> PLTATVDGIIQPMLKAYRIPGMAVAVLKDGKAHYFNYGVANRESGQRVSEQTLFEIGSVSKTLTATLGAYAAVKGGFELDDKVSQHAPWLKGSAFDGVTMAELATYSAGGLPLQFPDEVDSNDKMQTYYRSWSPVYPAGTHRQYSNPSIGLFGHLAANSLGQPFEQLMSQTLLPKLGLHHTYIQVPESAMANYAYGYSKEDKP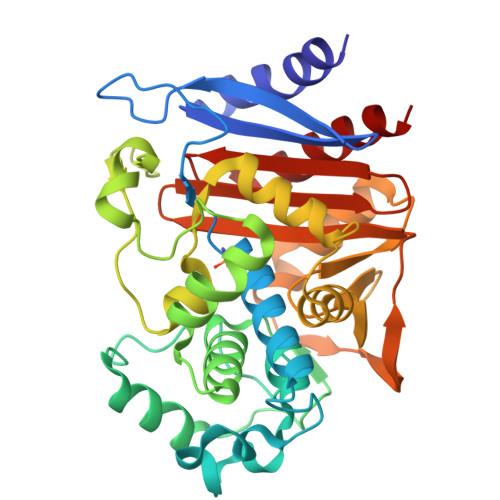IRATPGVLAAEAYGIKTGSADLLKFVEANMGYQGDAALKSAIALTHTGFHSVGEMTQGLGWESYDYPVTEQVLLAGNSPAVSFQANPVTRFAVPKAMGEQRLYNKTGSTGGFGAYVAFVPARGIAIVMLANRNYPIEARVKAAHAILSQLAE>GSSGSSGAEGTKLDDEFLDMERKIDVTNKVVAEILSKTTEYLQPNPAYRAKLGMLNTVSKIRGQVKTTGYPQTEGLLGDCMLKYGKELGEDSTFGNALIEVGESMKLMAEVKDSLDINVKQTFIDPLQLLQDKDLKEIGHHLKKLEGRRLDYDYKKKRVGKIPDEEVRQAVEKFEESKELAERSMFNFLENDVEQVSQLAVFIEAALDYHRQSTE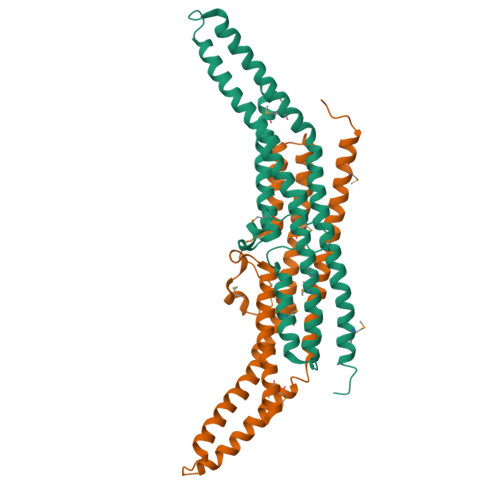ILQELQSKLQMRISAASSVPRREYK[2x]>[4x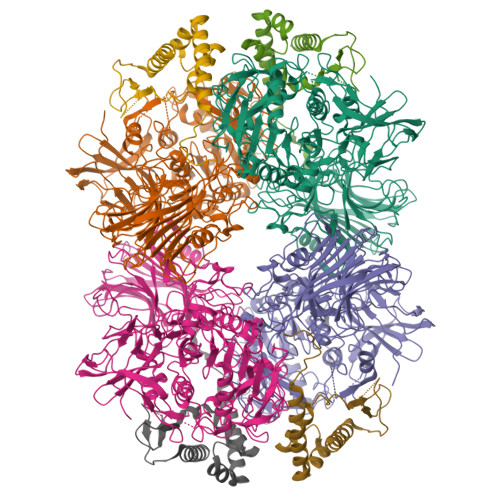]MKDIAIRGYCDRPSVATGETIRFYVSANETRGTFDAELVRLIHGDSNPAGPGYKEEAIKSDLEGQYPARFQRTQFGSYVEVADPDAGLQPDGAFSVHLFLWSTTPSRGRQGIASRWNDERQSGWNLAIEDGRVVFTIGDGSGATSSVVSDRPLFQQIWYSITGVYDPEKKQLRLYQKSVVNRTNSRFGLVVPLDSDCAVSADATVKAADSETSLLIAGLGEAAAQDGRTWCIAHYNGKVDAPKIYGCALGQDDAEKLSRGEIVRPISRLAHWDFSAGIGLNGIPTDHVVDASGYGHHGRCMNQPSRGSTGWNWDGHEENFIHCPEQYGALWFHEDCLDDCRWEKDFEFTVPEGLKSDFYAVKIRYEDTEDYIPFFVLPPRGTATAPILVIASTLSYLAYANEQIMHKADIGQAVAGHTPVLNENDVELHKNLSYYGLSTADGHIDGRGVQYTSWRRPIMNLRPKHRQGFGSIWELPADLHLIDWLNHNGFEYDVATEHDLNDQGAELLRRYKVVLTGSHPEYQTWANADAWEDYLADGGRGMYLAANGMYWIVEVHPEKPWVMEVRKELGVTAWEAPPGEYHYSTNGRRGGRFRGRARATQKIWGTGMSSFGFDHSGYFVQMPDSQDERVAWIMEGIDPEERIGDGGLVGGGAGGYELDRYDLALGTPPNTLLLASSVEHSVVYTVIPDDKAFPHPGMNGGEHPFVRADITYFSTANGGGMFATSSISWLGSLSWNDYDNNVSKMTKNVLNQFIKDEPAPRVKLAAALEHHHHHH;>[4x]MTEASESCVRDPSNYRDRSADWYAFYDERRRKEIIDIIDEHPEIVEEHAANPFGYRKHPSPYLQRVHNYFRMQPTFGRYYIYSEREWDAYRIATIREFGELPELGDERFKTEEEAMHAVFLRRIEDVRAELA>[2x]SMNYFVGNSLGVNLTGIEKAIINRLNLFKEMGRPAQCVFLSWNRYLYRNAQNYITSSDYINMYDFFQEATYLERNEPFDWLSYWTDECHYTLKHVENSHDFRIYDQERFLMYAHFQDPKYRILDYVNHFDSQRRKVKRDFYDVRGFLSCSRILVDKQQTLCEFFYNPEGDTKLEKYFSYKDGKPEVQKIIVYYANKQYFFNNETELGAFFIKQLYQHGDLFFSDRNVYTAPIFNLTPESIPVVAVLHSTHIKNIDALDSSPFKNVYKAMFENLSRYRAIIVSTEQQKLDVEKRINHTIPVVNIPVGYSETIDTPVQTLDQRSVKLISVARYSPEKQLHQQIELIKRLVSYVPKIELHMYGFGSESKKLNELIQKYGLENHVYLRGFLSNLDQEYSDAYLSLITSNMEGFSLALLESLAHGVPVISYDIKYGPNELITSDFNGYLITKNDEDALFDKVKYVIDHPEVQQRLSKGSLAKAQQYSKASLIKQWDQFVRLILEHHHHHH;> DSD

Two glycosyltransferases (GTases), SdgB and SdgA, are responsible for the glycosylation of S. aureus SDR proteins such as ClfA and ClfB. SdgB first appends N-acetyl­glucosamine (GlcNAc) moieties onto serine residues (O-glycosylation) within the SDR domain using uridine diphos­phate N-acetylglucosamine (UDP-GlcNAc) as a donor substrate. The subsequent addition of GlcNAc to the glycoproteins is catalyzed by the second enzyme, SdgA, yielding glycosylated SDR proteins in which each SD repeat is decorated with GlcNAc disaccharide moieties. The glycosylation of SDR proteins mediated by SdgA and SdgB protects SDR proteins from degradation by host proteases, thereby circumventing innate immune attack.

Despite the biological significance of these two glycosyltransferases involved in pathogenicity and avoidance of the host innate immune response, their structures and the molecular basis of their activity have not been investigated. This study reports the crystal structures of SdgB and SdgA from S. aureus as well as multiple structures of SdgB in complex with its substrates (for example UDP, N-acetylglucosamine or SDR peptides), products (glycosylated SDR peptides) or phosphate ions. In addition to the dimerization role, the inserted domain was found to serve as a binding platform for the SD repeats before and after glycosylation. Altogether, the extensive snapshots of SdgB complexes in multiple states provided a mechanistic insight into how SdgB recognizes and glycosylates the clustered serine residues in the SDR proteins.The envelope of Gram-negative pathogens, such as Acinetobacter baumannii and Pseudomonas aeruginosa, contains unique tripartite machineries that export noxious compounds from the cell. MacA-MacB-TolC contains similar components as the relatively well-characterized tripartite RND transporters AcrA-AcrB-TolC in E. coli and MexA-MexB-OprM in P. aeruginosa. However, the ABC protein MacB is unrelated to AcrB and MexB, which form large trimeric complexes in the plasma membrane, raising questions about the structure and domain organization of MacB in the tripartite efflux pump. Here, we present the crystal structure of MacB, and show that, by analogy to RND transporters, the MacB homodimer contains two large periplasmic domains (PLDs) that enable the interactions with the other components in this tripartite efflux pump.

MacB was purified and its crystal structure was solved at 3.4-Å resolution. MacB was crystallized in the presence of adenosine-5′-(β-thio)-diphosphate (ADPβS). The two NBDs are dimerized in a head-to-tail arrangement, and both subunits contribute conserved Walker A, Walker B and ABC signature motifs and residues to form two composite nucleotide-binding sites at the dimer interface. Electron density was observed in the difference Fourier map at the expected position for the nucleotide-binding site. Although the shape of the difference Fourier map is not optimally fitted by the ADPβS model, the phosphor and sulphur atoms of the bound ADPβS are clearly identified in the anomalous difference Fourier map (7σ, 0.013 electron Å−3). The binding of the adenine moiety of the nucleotide involves a π-stacking interaction with a conserved aromatic residue (Phe16) in the A-loop of the NBD. When MacB is compared with outward-facing structures of MsbA and Sav1866, which participate in alternating access mechanisms for these transporters, the overall structure provides a similar V-shape opening with access to the periplasm. However, the locations of these openings are different. The cavity in Sav1866 is present in the outer leaflet of the phospholipid bilayer, whereas the cavity in MacB is present in the periplasmic space. The TMD of MacB does not exhibit a distinct cavity in the membrane-embedded sections of the TMs, suggesting that a substrate-binding pocket might not exist in this part of MacB.

>[2x]MHHHHHHMTKQALLEVSNLVREFPAGESTIQILKGIDLTIYEGELVAIVGQSGSGKSTLMNILGCLDRPTSGSYKVNGQETGKLEPDQLAQLRREYFGFIFQRYHLLGDLSAEGNVEVPAVYAGVTPADRKQRATALLTELGLGTKTQNRPSQLSGGQQQRVSIARALMNGGDVILADEPTGALDSHSGVEVMRILRELNAAGHTIILVTHDMQVAKNATRIIEISDGEIISDRPNVPDQSLEEVKSDPDAAPALQNKQKKGKSISAWRSTLDRLSEAFQMALLSMNAHRMRTFLTMLGIIIGIASVVTVVALGNGSQQQILSNISSLGTNTITVFQGRGFGDNSKTANFKTLVPADADALMTQPYVSAVSPMVSTSKTMRYQQNEANATINGVSNDYFDVKGLVFKDGQTFDQRSVRDRSQDVVIDTNTQKQFFSDGTNPIGQVVLLGSVPARIIGIVEPQTSGMGSDDTLNVYMPYTTVMSRMLGQAHVRNIVVRINDKYSTSAAENAIVNLLTQRHGAQDIFTMNSDSIRQTIEKTTSTMTLLVSAIAVISLVVGGIGVMNIMLVSVTERTQEIGVRMAVGARQSDILQQFLIEAILVCLIGGVLGVLLSLGLGQLINKFAGGNFAVAYSTTSIVAAFVCSTLIGVVFGFLPAKNAAKLDPVAALSRE>MNSQNSQIQPQARYILPSFIEHSSFGVKESNPYNKLFEERIIFLGVQVDDASANDIMAQLLVLESLDPDRDITMYINSPGGGFTSLMAIYDTMQYVRADIQTVCLGQAASAAAVLLAAGTPGKRMALPNARVLIHQPSLSGVIQGQFSDLEIQAAEIERMRTLMETTLARHTGKDAGVIRKDTDRDKILTAEEAKDYGIIDTVLEYRKLSAQTA[14x];>[14x]MSQVTDMRSNSQGLSLTDSVYERLLSERI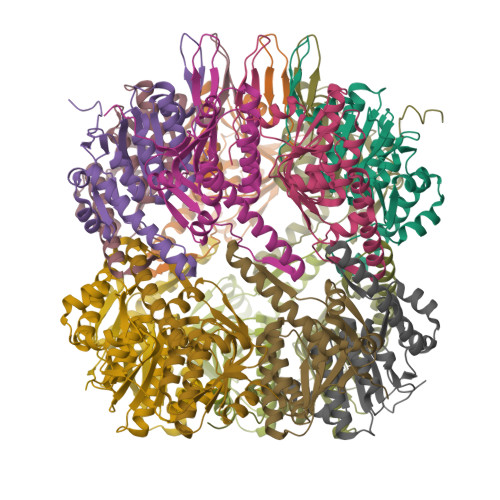IFLGSEVNDEIANRLCAQILLLAAEDASKDISLYINSPGGSISAGMAIYDTMVLAPCDIATYAMGMAASMGEFLLAAGTKGKRYALPHARILMHQPLGGVTGSAADIAIQAEQFAVIKKEMFRLNAEFTGQPIERIEADSDRDRWFTAAEALEYGFVDHIITRAHVNGEAQ[(~{E},4~{S})-4-azanyl-3-oxidanylidene-pent-1-enyl] dihydrogen phosphate | C5 H10 N O5 P | 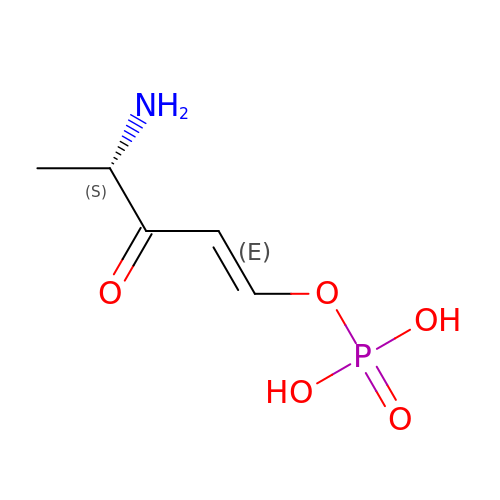RTVKPJRIOVZREZ-ZPYNKGFJSA-N>MSFRKRGEILNDRGSGLRGPLLRGPPRTSSTPLRTGNRRAPGNVPLSDTTARLKKLNIADESKTKMGLDSSHVGVRPSPATSQPTTSTGSADLDSILGHMGLPLGNSVLVEEQSTTEFHSILGKLF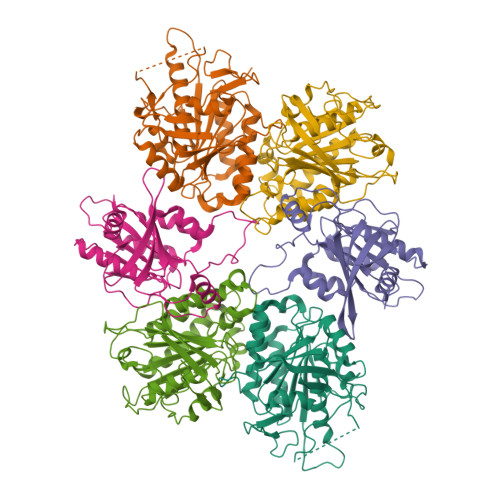AAQGIVHNRISDSSADKTRNGDTHVIVLSLNQMFAKELPGIYKGSRKQMKKNLISEEESKVTVQNLNETQRSTPSRYKDLKIAWKYKLADEKRLGSPDRDDIQQNSEYKDYNHQFDITTRLMPAPIASELTFIAPTQPVSTILSQIEQTIKRNDKKLIRIVIPSLLHPAMYPPKMFESSEIIGLMHGVRSLVKKYYERVVLFASISIDIITPPLLVLLRNMFDSVINLEPFNQEMTEFLERVYKSQPGKIQHGLVHILKLPVFTDRGEMRVLKSEWAFKNGRKKFEIEQWGIPVDDAEGSAASEQSHSHSHSDEISHNIPAKKTKISLDY[2x];>[2x]MASSSHNPVILLKRILSLTESSPFILCLDSIAQTSYKLIQEFVHQSKSKGNEYPIVYISFETVNKPSYCTQFIDATQMDFVHLVKQIISYLPAATATQAKKHMVIIDSLNYISTEYITRFLSEIASPHCTMVATYHKDIKDENRTVIPDWNNNYPDKLTLLQFMATTIVDIDVVLTGTLDTEEVSELLNEFRIPRGLNNDIFQLRLVNKRKSGRSLEYDFIVNSNTHEYELLSTTKQEEESSSNGLETPEMLQGLTTFNLGTSNKQKLAKDQVALPFLEAQSFGQGGAIVYEYEKDDDYDEEDPYEDPF;>[2x]MGSVQRQDLVLFSDQSVLPAHFFQDSNSHNLFFITHQSCTQPLWMINALVETHVLGSPSSLNESSSSMLPSSTRSHAVLASFIHEQNYFTNSLNKLKIPSNNYNVLDFLSDFIVNNIHNKPRDKILSDVLAKFSAAIQNNPTDTIVIIEQPELLLSLVSGLTCSELNNKFITPLLRQCKVLIIVSNSDIFNIDEYDASVHSSNLQNFYKSSFIKSMINLNLNPLKTGFAKDVTGSLHVCRGGAPIATSNTSLHVVENEYLYLNEKESTKLFYR> MYLLIVFLPLLGSSVAGFFGRFLGSEGSAIMTTTCVSFSSILSLIAFYEVALGASACYLRIAPWISSEMFDASWGFLFDSLTVVMLIVVTFISSLVHLYSISYMSEDPHSPRFMCYLSIFTFFMLMLVTGDNFLQLFLGWEGVGLASYLLIHFWFTRLQADKAAIKAMLVNRVGDFGLALGILGCFTLFQTVDFSTIFACASVPRNSWIFCNMRLNAISLICILLFIGAVGKSAQIGLHTWLPDAMEGPTPVSALIHAATMVTAGVFMIARCSPLFEYSPTALIVITFAGAMTSFLAATTGILQNDLKRVIAYSTCSQLGYMIFACGISNYSVSVFHLMNHAFFKALLFLSAGSVIHAMSDEQDMRKMGGLASSFPLTYAMMLIGSLSLIGFPFLTGFYSKDVILELAYTKYTISGNFAFWLGSVSVLFTSYYSFRLLFLTFLVPTNSFGRDISRCHDAPIPMAIPLILLALGSLFVGYLAKDMMIGLGTNFWANSLLVLPKNEILAESEFAAPTIIKLIPILFSTLGAFVAYNVNLVADQFQRAFQTSTFCNRLYSFFNKRWFFDQVLNDFLVRSFLRFGYEVSFEALDKGAIEILGPYGISYTFRRLAERISQLQSGFVYHYAFAMLLGLTLFVTFFCMWDSLSSWVDNRLSFILIVSSFYTKSSQE;> MLEHFCECYFNLSGLILCPVLGSIILLFIPNSRIRLIRLIGLCASLITFLYSLVLWIQFDSSTAKFQFVESLRWLPYENINFYLGIDGISLFFVILTTFLIPICILVGWSGMRSYGKEYIIAFLICEFLMIAVFCMLDLLLFYVFFESVLIPMFIIIGVWGSRQRKIKAAYQFFLYTLLGSLFMLLAILLILFQTGTTDLQILLTTEFSERRQIFLWIAFFASFAVKVPMVPVHIWLPEAHVEAPTAGSVILAGILLKFGTYGFLRFSIPMFPEATLCFTPFIYTLSAIAIIYTSLTTLRQIDLKKIIAYSSVAHMNLVTIGMFSLNIQGIGGSILLMLSHGLVSSALFLCVGVLYDRHKTRLVRYYGGLVSTMPNFSTIFFFFTLANMSLPGTSSFIGEFLILVGAFQRNSLVATLAALGMILGAAYSLWLYNRVVSGNLKPDFLHKFSDLNGREVFIFIPFLVGLVWMGVYPKVFLDCMHTSVSNLVQHGKFH;> MALRNAILRHLRVPVQTLGLNQSKIGFLGTIRSFSSHDDHLSREAVVDRVLDVVKSFPKVDPSKVTPEVHFQNDLGLDSLDTVEIVMAIEEEFKLEIPDKEADKIDSCSLAIEYVYNHPMSS;> MGGGDHGHGAEGGDFRAKVWSMTGGPNCRPKHWRRNTAIAMFGVFLVCIPIAKLSAKLEQRPHMPVRPIPSQIWCKNFGTKDDYEKEH;> MPSTQSLTVAAKTLRNRIFSRSGSTSAGPSRWATPGHEERPKGYFMNRTPPAPGQSRKWEDWELPCYITSFLTIVILGVGLNAKPDLSIETWAHQKALERLEMEKLATAGDSSD;> MGFIMEFAENLVLRLMENPEERDRKAREHIYEMHERCKKIKEMWALPIRPYGFWTFERHNAQLRWDPQISQVAGRRDPYDDLLEDNYTPPSSSSS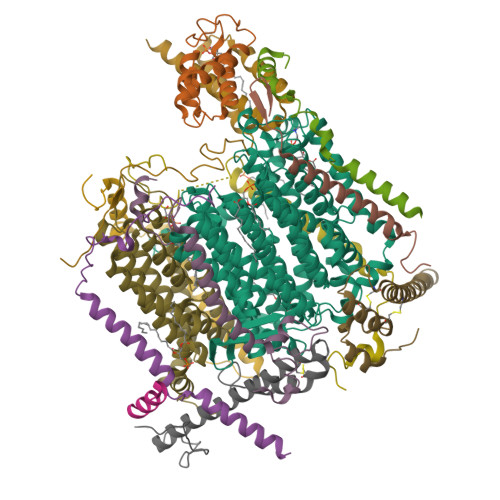SSD;> MGGGGHGGGITYKGVTVHTPKTWHTVTGKGLCAVMWFWILYRAKQDGPVVMGWRHPWDGHGDHGHGDHH;> MAKPLGTTGEFFRRRDEWRKHPMLSNQMRHALPGIGIGVGAFCVYLVGEQIYSKLMAPSSQSSHQKQPAPSH;> MAGRLSGVASRIMGGNGVVARSVGSSLRQRAGMGLPVGKHIVPDKPLSVNDELMWDNGTAFPEPCIDRIADTVGKYEALAWLSGGLGFFVGLGLLAVLNDKASKVPFTPRVYPYDNLRVELGGEP;> MGGGMETNKNKFIEDWGSARENLEHNFRWTRRNFALIGIFGIALPIIVYKGIVKDFHMQDEDAGRPHRKFL;> MSGVSTAAYFARRAAQKERVRILYRRALKDTLNWAVHRHIFYRDASDLREKFNVNQDVEDVDRIDKLIAHGEAEYNKWRHPDPYIVPWAPGGSKFCRNPTPPAGIEIVYNYGLEDNP;> MEVPGSSKKMIATQEEMSAAKIALGSRDMCAHLLIPLNKCRQAEFYLPWKCEDERHVYEKCEYELVMERMLAMKKIREEEALAKQNKLQGNAAVPLIPKTANA;> MGRKKGLPEFEESAPDGFDPENPYKDPVAMVEMREHIVREKWIQIEKAKILREKVKWCYRVEGVNHYQKCRHLVQQYLDSTRGVGWGKDHRPISLHGPKPEAVEAE> MLNGEDFVEHNDILSSPAKSRNVTPKRVDPHGERQLRRIHSSKKNLLERISLVGNERKNTSPDPALKPKTPSKAPRKRGRPRKIQEELTDRIKKDEKDTISSKKKRKLDKDTSGNVNEESKTSNNKQVMEKTGIKEKREREKIQVATTTYEDNVTPQTDDNFVSNSPEPPEPATPSKKSLTTNHDFTSPLKQIIMNNLKEYKDSTSPGKLTLSRNFTPTP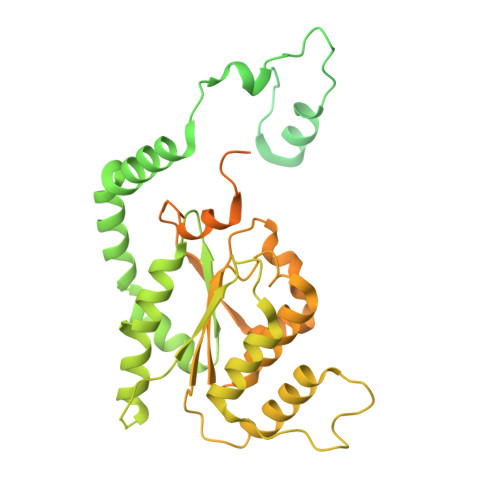VPKNKKLYQTSETKSASSFLDTFEGYFDQRKIVRTNAKSRHTMSMAPDVTREEFSLVSNFFNENFQKRPRQKLFEIQKKMFPQYWFELTQGFSLLFYGVGSKRNFLEEFAIDYLSPKIAYSQLAYENELQQNKPVNSIPCLILNGYNPSCNYRDVFKEITDLLVPAELTRSETKYWGNHVILQIQKMIDFYKNQPLDIKLILVVHNLDGPSIRKNTFQTMLSFLSVIRQIAIVASTDHIYAPLLWDNMKAQNYNFVFHDISNFEPSTVESTFQDVMKMGKSDTSSGAEGAKYVLQSLTVNSKKMYKLLIETQMQNMGNLSANTGPKRGTQRTGVELKLFNHLCAADFIASNEIALRSMLREFIEHKMANITKNNSGMEIIWVPYTYAELEKLLKTVLNTL Several clusters of these genes showed sequence similarity with the chaperone/usher (CU) pathway, which is conserved in Gram negative bacteria and involved in the assembly of extracellular fimbriae. One of these clusters, encoded by the cupB operon, is unique as it contains a non-chaperone-usher gene product, CupB5, which is related to the TpsA-like substrates of two-partner secretion (TPS) systems. The CupB4 chaperone was shown to be associated with the tip adhesin CupB6, which is larger than classical adhesive tip subunits and displays only limited sequence identity with other CU subunits. In this paper we describe the crystal structure of the tip adhesin CupB6.

The crystals belong to C2 space group and the asymmetric unit consists of eight molecules composed from two up-down-up-down tetramers. The molecular mass of CupB6dscB1 in solution was determined to be 39.5 kDa, which is consistent with a monomer. Each molecule consists of two domains comprising a putative tip adhesin (residues; 1–202) and the pilin domain (202–343). The pilin domain conforms to the classical Ig-like fold of other chaperone-usher pilin domains with a C-terminal β strand (strand G), provided by the NTE of CupB1 located at the C-terminus. Five alternating residues comprising glycine or large hydrophobic residues from the self-complementing G strand (G351, V353, F355, G357 and I359) are positioned to interact with the five pockets of the subunit groove. The adhesin domain of CupB6 is 205 amino acid residues in length and is significantly larger than typical adhesion domains of the chaperone-usher family, which are usually between 150 and 180 residues. One unique feature in the CupB6 structure is a surface-exposed polyproline helix (199PPPPPIP205) at the C-terminus of the adhesion domain. Adjacent to this is a shorter sequence (17LPWR19) that also adopts PPII helical secondary structure despite containing only one central proline. Adjacent to the PPII helix in CupB6 is a shallow pocket delineated by hydrophobic residues V21, L25, F36 and I204, which further suggests a role in receptor binding. The lack of a convincing binding pocket at the tip of the CupB6 adhesin domain would suggest it recognizes its receptor using an alternative surface.

>[8x]MALNEVALNCSFDNGKGLPWRVVNELTSGTAKGTVLFARPVSLFLNYKPQASQEAHELVIGGNWSGVGYPGPYGTVASDVKGIGYRISVDAQDGVKRVIPVDNQPHALDKRVTSFSGSTTSDYLQELVLTVDPGELPAGDLKVTSVSGSATLNLWAVDRLKGEASIGSVLAVPADNYPTGVCRKPYSLIGPASIAIGGGPPPPPIPKKCKVEVGREINVKLGSVALKNFPRVNDTSTERSFDISLSECAALAKPEIAFRDKYVSAQQADPTILSLKSGGAAGFGIVVKNGLDQQRIRFDGTPYPMRRVGDSADLPLSAAYIRIGAEGELKAGVADGAAEFTFTFPSDNKVDGIVNFSGNITELEHHHHHH2-(4-methylphenyl)-5,7-bis(oxidanyl)chromen-4-one 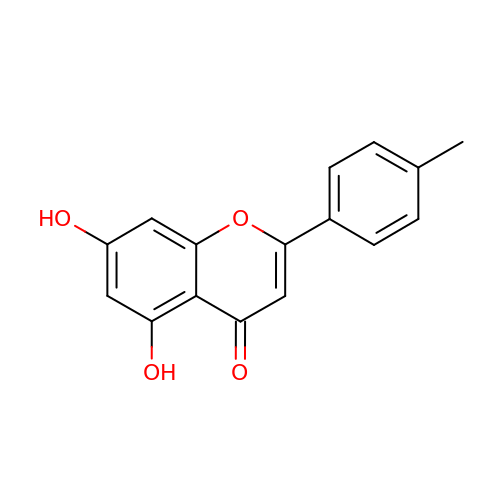| C16 H12 O4 | PXFZXOXUQVAZOV-UHFFFAOYSA-N>[2x]MRSLGANMAAALRAAGVLLRDPLASSSWRVCQPWRWKSGAAAAAVTTETAQHAQGAKPQVQPQKRKPKTGILMLNMGGPETLGDVHDFLLRLFLDRDLMTLPIQNKLAPFIAKRLTPKIQEQYRRIGGGSPIKIWTSKQGEGMVKLLDELSPNTAPHKYYIGFRYVHPLTEEAIEEMERDGLERAIAFTQYPQYSCSTTGSSLNA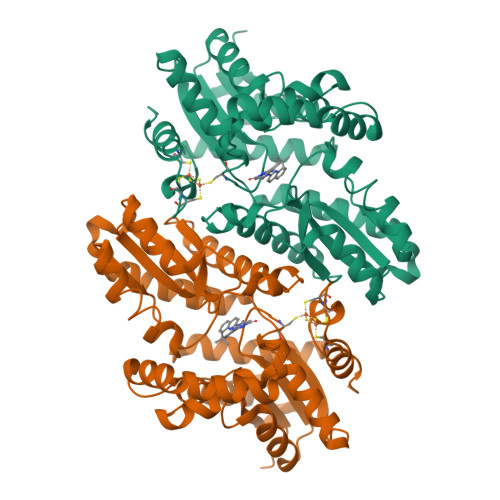IYRYYNQVGRKPTMKWSTIDRWPTHHLLIQCFADHILKELDHFPLEKRSEVVILFSAHSLPMSVVNRGDPYPQEVSATVQKVMERLEYCNPYRLVWQSKVGPMPWLGPQTDESIKGLCERGRKNILLVPIAFTSDHIETLYELDIEYSQVLAKECGVENIRRAESLNGNPLFSKALADLVHSHIQSNELCSKQLTLSCPLCVNPVCRETKSFFTSQQL> PELPEVETIRRTLLPLIVGKTIEDVRIFWPNIIRHPRDSEAFAARMIGQTVRGLERRGKFLKFLL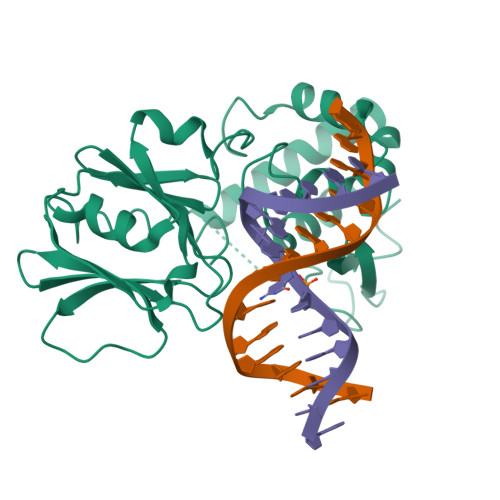DRDALISHLRMEGRYAVASALEPLEPHTHVVFCFTDGSELRYRDVRKFGTMHVYAKEEADRRPPLAELGPEPLSPAFSPAVLAERAVKTKRSVKALLLDCTVVAGFGNIYVDESLFRAGILPGRPAASLSSKEIERLHEEMVATIGEAVMKGGNHHLYVYGRQGNPCKRCGTPIEKTVVAGRGTHYCPRCQR>GTSSMADIGSGEFKIVKRSDARQIVNSEAVVDSATSKFVSLLFGYSKNSLRDRKDQLMQYCDVSFQTQAMRMFNENIRQFVDKVRAEAIISSNIQREKVKNSPLTRLTFFITI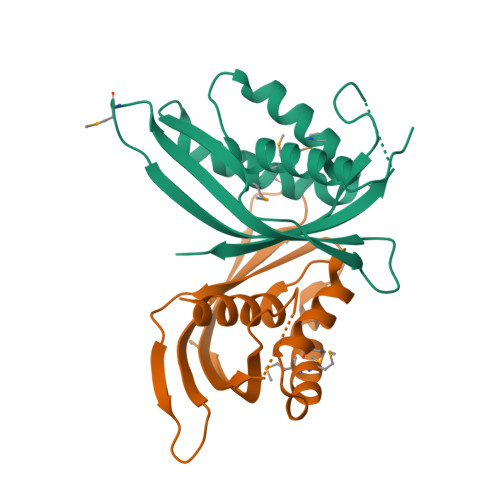KITPDTMENYEYITKKQVTIYYDFARGNSSQENLIINPFGFKVFDIQITDLQN[4x]> AECSVDIQGNDQMQFNTNAITVDKSCKQFTVNLSHPGNLPKNVMGHNWVLSTAADMQGVVTDGMASGLDKDYLKPDDSRVIAHTKLIGSGEKDSVTFDVS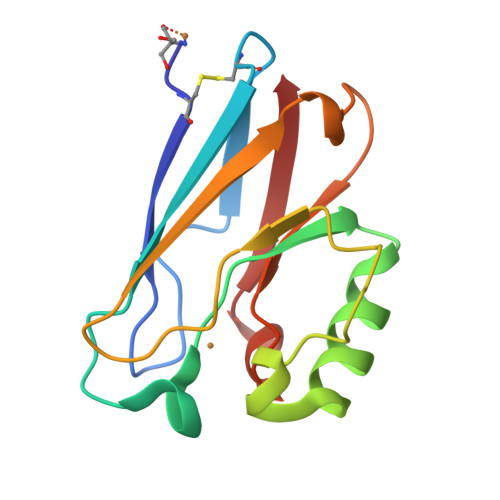KLKEGEQYMFFDTFPGHSALIKGTLTLK>GSGEEVSEEGFQIPATITERYKVGRTIGDGNFAVVKECVERSTAREYALKIIKKSKCRGKEHMIQNEVSILRRVKHPNIVLLIEEMDVPTELYLVMELVKGGDLFDAITSTNKYTERDASGMLYNLASAIKYLHSLNIVHRDIKPENLLVYE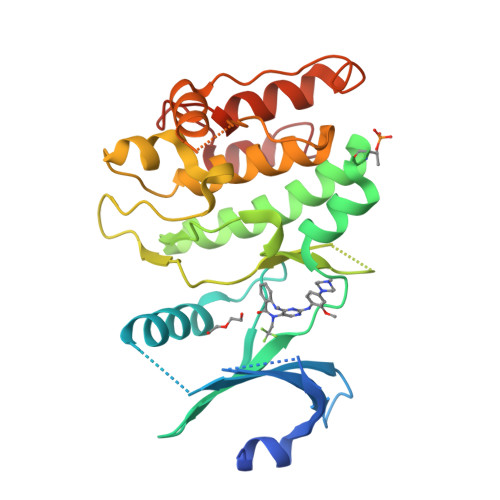HQDGSKSLKLGDFGLATIVDGPLYTVCGTPTYVAPEIIAETGYGLKVDIWAAGVITYILLCGFPPFRGSGDDQEVLFDQILMGQVDFPSPYWDNVSDSAKELITMMLLVDVDQRFSAVQVLEHPWVND[2x]> SNAMKKIAVFASGNGSNFQVIAEEFPVEFVFSDHRDAYVLERAKQLGVLSYAFELKEFESKADYEAALVELLEEHQIDLVCLAGYMKIVGPTLLSAYEGRIVNIHPAYLPEFPG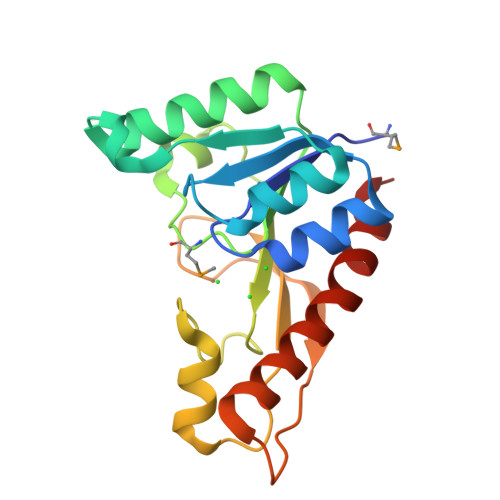AHGIEDAWNAGVGQSGVTIHWVDSGVDTGQVIKQVRVPRLADDTIDRFEARIHEAEYRLYPEVVKALFTD>MHLKIVCLSDEVREMYKNHKTHHEGDSGLDLFIVKDEVLKPKSTTFVKLGIKAIALQYKSNYYYKCE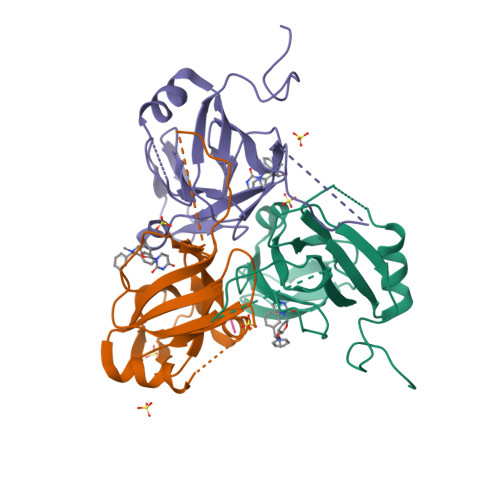KSENKKKDDDKSNIVNTSFLLFPRSSISKTPLRLANSIGLIDAGYRGEIIAALDNTSDQEYHIKKNDKLVQLVSFTGEPLSFELVEELDETSRGEGGFGSTSNNKYEAHHHHHH[3x];> GHG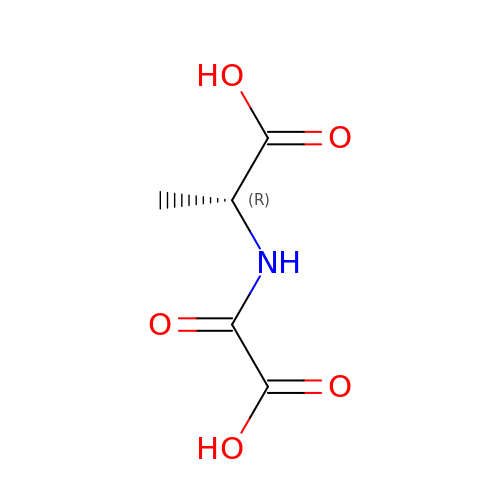(2~{R})-2-(carboxycarbonylamino)propanoic acid | C5 H7 N O5 | TZPZMVZGJVYAML-UWTATZPHSA-N> GQSGSSGSGSN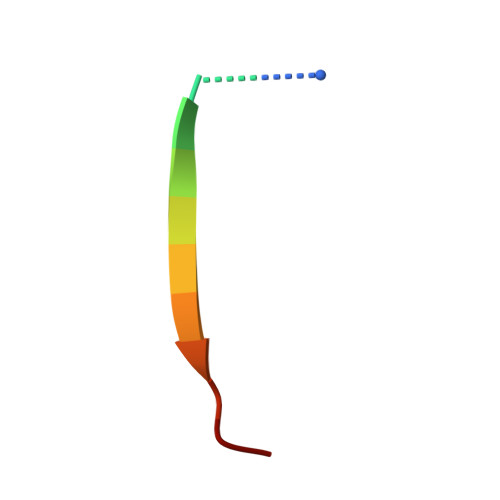GD> MADNQQRCELKLIASPGSWRLYSARKIDERFKSYEQKIFQRDRYTCQFCGFQARLYQDIVNLDGDYTNNRLSNLVTACCFCAQCFFVESVGVGGYGGGTLIYLPELTQAELNSLCHVLFCAITNDTGYKSSAQNIYRSFKFRSQIVEEKFGEGTSDPAIFGQLMIDSGVNSEEIREKLFKNIRL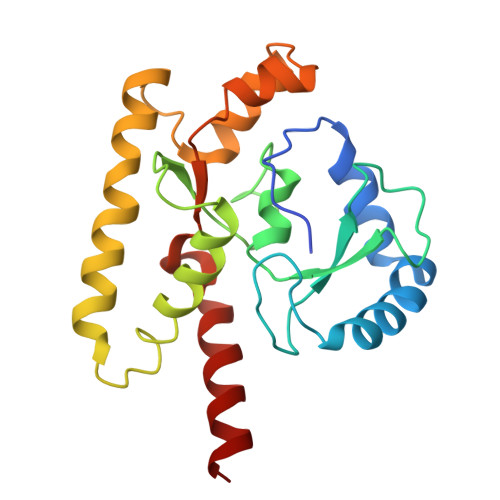LPSRAKFRKQIEKWAASALEEIAD The response regulator VbrR from Vibrio parahaemolyticus, a member of the OmpR/PhoB family, regulates virulence and antibiotic resistance genes. VbrR is a member of the OmpR/PhoB family and contains an N-terminal receiver domain (RD) and a C-terminal DNA-binding domain (DBD), connected by a flexible linker, and can directly bind with the promoter region of exsC to mediate its downregulation. The VbrK/VbrR TCS is activated by host-derived nitrite during infection, which leads to the downregulation of Type-3 secretion system-1 (T3SS1) via repression of its positive regulator exsC for maximal virulence. In the cell or solution, VbrR proteins exist mainly as inhibitory dimers formed through the DBD, and phosphorylation of RDs allows the formation of RD dimers, which in turn changes the conformation of the DBD from an inhibitory state to an active state.

We purified and crystallized the RD protein in the presence of BeF 3 – and solved the corresponding structure to 2.80 Å. The asymmetric unit contains fourteen RD molecules, comprising four dimers (AB, CD, EF, and GH) and six monomers (I to N). However, the BeF 3 – molecule only binds to molecules A, B and E, among which molecules A and B form a homodimer. The AB homodimer superimposes very well with the RD domain structure within the VbrR-DNA complex (RMSD is 0.92 Å), and the dimer interface is composed of α4-β5-α5 from both protomers, both of which represent an active dimer conformation. The homodimer interaction surface is maintained mainly by four intermolecular salt bridges formed between residues Asp91, Asp96, Arg110 and Arg112 from each protomer, and all these residues are highly conserved among members of the OmpR/PhoB subfamily. The other three dimers (CD, EF, and GH) in the asymmetric unit also adopt an active conformation similar to that of AB, even without BeF 3 – binding, probably due to crystal packing or high protein concentration. The BeF 3 – molecule is noncovalently bound to the active site Asp51, where it occupies four coordination sites with residues Thr78, Lys100, Gln53, and Mg 2+. Mg 2+ forms five coordinates with BeF 3 –, residues Glu9, Asp10, and Gln53. Interestingly, six molecules (I to N) exist as monomers in the asymmetric unit. In particular, the residue Tyr97 adopting an inward-facing conformation in the active dimer changes to an outward-facing conformation in all the monomers.

>[14x]MKQTLLLVEDDKNLADGLLVSLEQAGYECLHVERIADVEPQWKKADLVILDRQLPDGDSVQHLPEWKKIKDVPVILLTALVTVKDKVAGLDSGANDYLTKPFAEAELFARIRAQLRA>G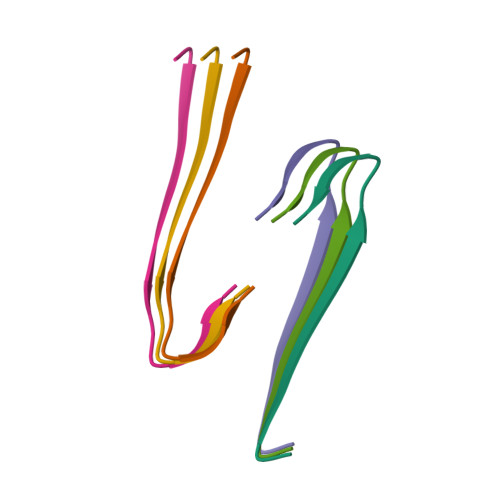LFDIIKKVASVIGGL[6x]L-CAPTOPRIL | C9 H15 N O3 S | 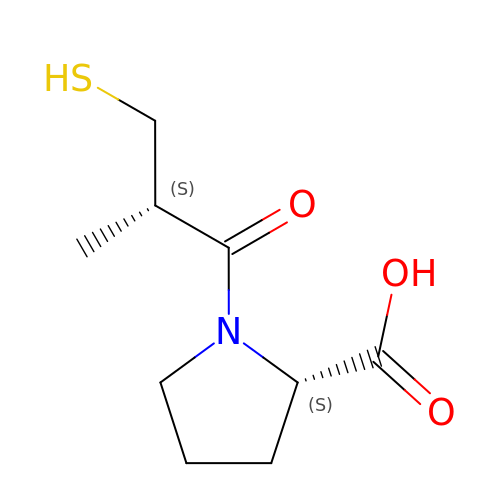FAKRSMQSSFJEIM-RQJHMYQMSA-N[(S)-(naphthalen-1-yl)(octadecyloxy)methyl]phosphonic acid | C29 H47 O4 P | 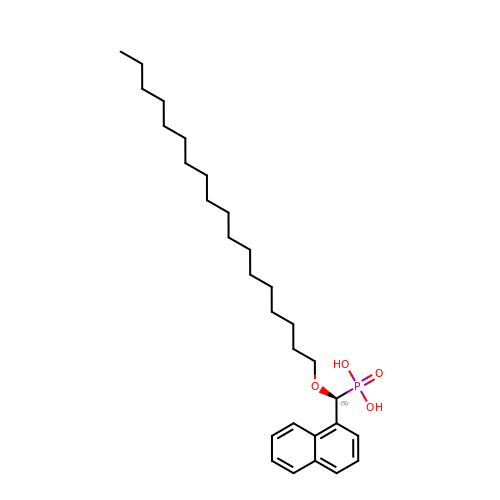IIAOXWLLPSQBBO-LJAQVGFWSA-N>MAKAHIELTINGHPVEALVEPRTLLIHFIREQQNLTGAHIGCDTSHCGACTVDLDGMSV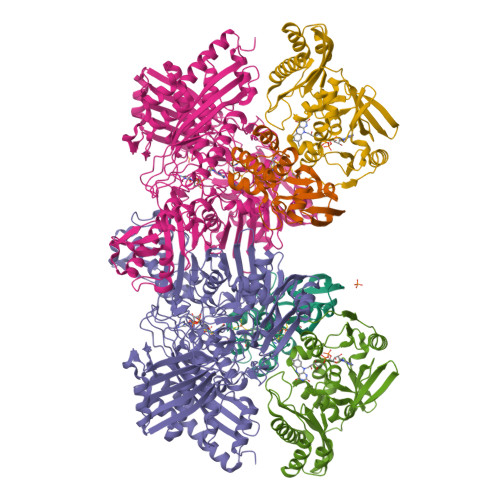KSCTMFAVQANGASITTIEGMAAPDGTLSALQEGFRMMHGLQCGYCTPGMIMRSHRLLQENPSPTEAEIRFGIGGNLCRCTGYQNIVKAIQYAAAKINGVPFEEAAE[2x];>MNIQTTVEPTSAERAEKLQGMGCKRKRVEDIRFTQGKGNYVDDVKLPGMLFGDFVRSSHAHARIKSIDTSKAKALPGVFAVLTAADLKPLNLHYMPTLAGDVQAVLADEKVLFQNQEVAFVVAKDRYVAADAIELVEVDYEPLPVLVDPFKAMEPDAPLLREDIKDKMTGAHGARKHHNHIFRWEIGDKEGTDATFAKAEVVSKDMFTYHRVHPSPLETCQCVASMDKIKGELTLWGTFQAPHVIRTVVSLISGLPEHKIHVIAPDIGGGFGNKVGAYSGYVCAVVASIVLGVPVKWVEDRMENLSTTSFARDYHMTTELAATKDGKILAMRCHVLADHGAFDACADPSKWPAGFMNICTGSYDMPVAHLAVDGVYTNKASGGVAYRCSFRVTEAVYAIERAIETLAQRLEMDSADLRIKNFIQPEQFPYMAPLGWEYDSGNYPLAMKKAMDTVGYHQLRAEQKAKQEAFKRGETREIMGIGISFFTEIVGAGPSKNCDILGVSMFDSAEIRIHPTGSVIARMGTKSQGQGHETTYAQIIATELGIPADDIMIEEGNTDTAPYGLGTYGSRSTPTAGAATAVAARKIKAKAQMIAAHMLEVHEGDLEWDVDRFRVKGLPEKFKTMKELAWASYNSPPPNLEPGLEAVNYYDPPNMTYPFGAYFCIMDIDVDTGVAKTRRFYALDDCGTRINPMIIEGQVHGGLTEAFAVAMGQEIRYDEQGNVLGASFMDFFLPTAVETPKWETDYTVTPSPHHPIGAKGVGESPHVGGVPCFSNAVNDAYAFLNAGHIQMPHDAWRLWKVGEQLGLHV[2x];>MIPGSFDYHRPKSIADAVALLTKLGEDARPLAGGHSLIPIMKTRLATPEHLVDLRDIGDLVGIREEGTDVVIGAMTTQHALIGSDFLAAKLPIIRETSLLIADPQIRYMGTIGGNAANGDPGNDMPALMQCLGAAYELTGPEGARIVAARDYYQGAYFTAIEPGELLTAIRIPVPPTGHGYAYEKLKRKIGDYATAAAAVVLTMSGGKCVTASIGLTNVANTPLWAEEAGKVLVGTALDKPALDKAVALAEAITAPASDGRGPAEYRTKMAGVMLRRAVERAKARAKN[2x]>[2x]MAHSSATAGPQADYSGEIAELYDLVHQGKGKDYHREAADLAALVRRHSPKAASLLDVACGTGMHLRHLADSFGTVEGLELSADMLAIARRRNPDAVLHHGDMRDFSLGRRFSAVTCMFS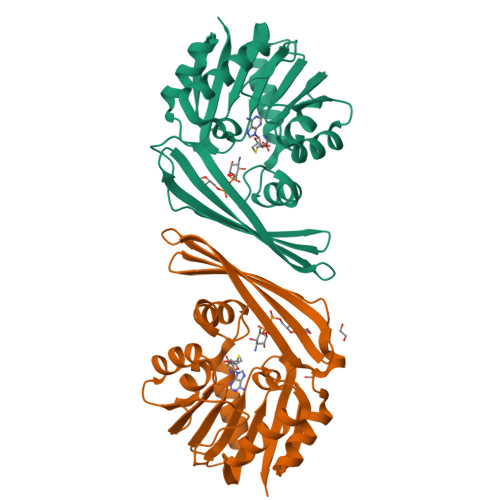SIGNLAGQAELDAALERFAAHVLPDGVVVVEPWWFPENFTPGYVAAGTVEAGGTTVTRVSHSSREGEATRIEVHYLVAGPDRGITHHEESHRITLFTREQYERAFTAAGLSVEFMPGGPSGRGLFTGLPGAKGETRLEHHHHH>MTSAEMTSPNNNSEHQA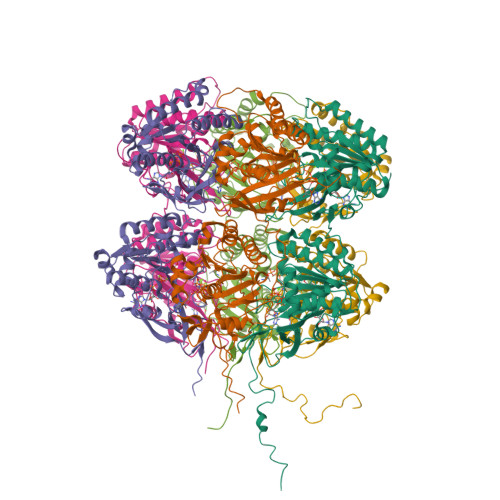IAKMRTMIEGFDDISHGGLPIGRSTLVSGTSGTGKTLFSIQFLYNGIIEFDEPGVFVTFEETPQDIIKNARSFGWDLAKLVDEGKLFILDASPDPEGQEVVGGFDLSALIERINYAIQKYRARRVSIDSVTSVFQQYDASSVVRRELFRLVARLKQIGATTVMTTERIEEYGPIARYGVEEFVSDNVVILRNVLEGERRRRTLEILKLRGTSHMKGEYPFTITDHGINIFPLGAMRLTQRSSNVRVSSGVVRLDEMCGGGFFKDSIILATGATGTGKTLLVSRFVENACANKERAILFAYEESRAQLLRNAYSWGMDFEEMERQNLLKIVCAYPESAGLEDHLQIIKSEINDFKPARIAIDSLSALARGVSNNAFRQFVIGVTGYAKQEEITGLFTNTSDQFMGAHSITDSHIATITDTIILLQYVEIRGEMSRAINVFKMRGSWHDKAIREFMISDKGPDIKDSFRNFERIISGSPTRITVDEKSELSRIVRGVQEKGPES[6x]3-pentyl-2-[(pyridin-2-ylmethyl)sulfanyl]-7-(pyrrolidin-1-ylcarbonyl)quinazolin-4(3H)-one 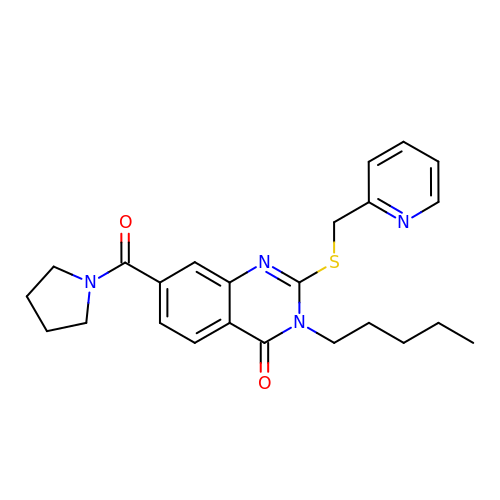| C24 H28 N4 O2 S | DSTQURGOCGYFAN-UHFFFAOYSA-N>MHSLQNVIPQQQAHIAELQVYNNKLERDLQNKIGSLTSSIEWYLRSMELDPEIKA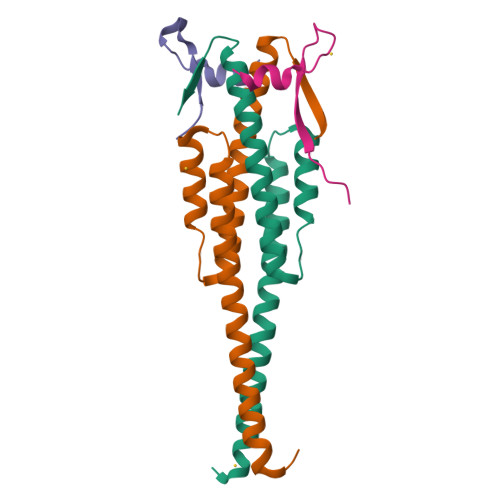DIEQQINSIDAINPLHAFDDLESVIRNLISDYDKLFLMFKGLIQRSNYQYSFGSE[2x];>APKRERKTIRIRDPNQGGKDITEEIMSG[2x]>SMLPNRMALSRQTEDQLKKLKGYTGITPNIAARLAFFRSVESEFRYSPERDSKKLDGTLVLDKITWLGETLQATELVLKMLYPQLEQKALIKAWAA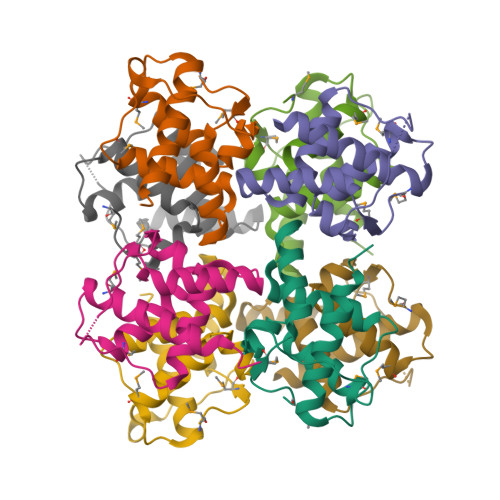HVEDGIAALRNHK[16x]> XPLVVA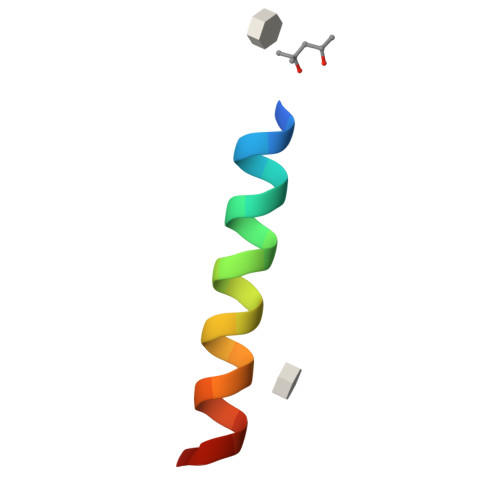ASIIAILHLALWILDRLX>MKPALVVVDMVNEFIH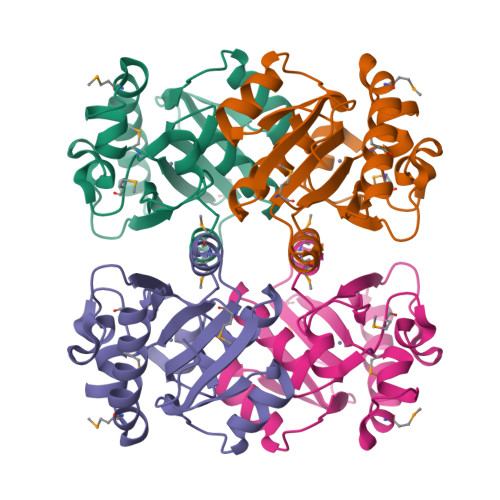GRLATPEAMKTVGPARKVIETFRRSGLPVVYVNDSHYPDDPEIRIWGRHSMKGDDGSEVIDEIRPSAGDYVLEKHAYSGFYGTNLDMILRANGIDTVVLIGLDADICVRHTAADALYRNYRIIVVEDAVAARIDPNWKDYFTRVYGATVKRSDEIEGMLQEDQIET[2x]> MSPEEWTYLVVLLISIPIGFLFKKAGPGLKRWGAAAVGLGLTLFTCGPHTLHSLVTILGTWALIQAQPCSCHALALAWTFSYLLFFRALSLLGLPTPTPFTNAVQLLLTLKLVSLASEVQDLHLAQRKEMASGFSKGPTLGLLPDVPSLMETLSYSYCYVGIMTGPFFRYRTYLDWLEQPFPGAVPSLRPLLRRAWPAPLFGLLFLLSSHLFPLEAVREDAFYARPLPARLFYMIPVFFAFRMRFYVAWIAAECGCIAAGFGAYPVAAKARAGGGPTLQCPPPSSPEKAASLEYDYETIRNIDCYSTDFCVRVRDGMRYWNMTVQWWLAQYIYKSAPARSYVLRSAWTMLLSAYWHGLHPGYYLSFLTIPLCLAAEGRLESALRGRLSPGGQKAWDWVHWFLKMRAYDYMCMGFVLLSLADTLRYWASIYFCIHFLALAALGLGLALGGGSPSRRKAASQPTSLAPEKLREELEACGIENLYFQ

Membrane-bound O-acyltransferase (MBOAT) 7 acylates lyso-phosphatidylinositol (lyso-PI) with arachidonyl-CoA. To adjust membrane properties according to need and to store specific fatty acids as precursors for bioactive lipids, cells remodel the phospholipid acyl chains in enzymatic reactions known as the Lands cycle. MBOAT7 mutations cause brain developmental disorders, and reduced expression is linked to fatty liver disease. Here, we report the structure and a model for the catalytic mechanism of human MBOAT7.

To enable biochemical and structural analyses of human MBOAT7, we purified recombinantly expressed enzyme in detergent and reconstituted it into amphipol PMAL-C8. We used single-particle cryo-EM to obtain a density map of MBOAT7 at an overall resolution of ~3.7 Å, allowing us to build a model of the entire protein except the C-terminal region (442–472), which was not visible and presumably disordered. MBOAT7 comprises 11 transmembrane (TM) helical segments, connected by short intervening helices (IH) and loops. The monomeric protein occupies a space of ~36 × 58 × 28 Å, embedded in the membrane, resembling the shape of a saddle. TM8, containing the putative catalytic His356 residue, resides in the cavity between the two TM bundles. TM8 exhibits weaker density than the other TMs, indicating flexibility or multiple conformations in the apo state of the enzyme (TM8 density shown in two σ values). A tunnel twists through MBOAT7, connecting the cytoplasmic and the ER lumenal sides of the enzyme, with the active site located in the middle of this tunnel. In MBOAT7, the lateral opening of the tunnel has an extended channel that branches off to the lumenal leaflet of the ER membrane. In contrast, TM helices 1 and 2 of MBOAT7 occlude the equivalent lateral gate region. Compared with other MBOAT structures, our cryo-EM structure of MBOAT7 is distinct, inasmuch as TM6 is divided into two short helices linked by two evolutionarily conserved proline residues that are not found in MBOATs 1, 2, or 5.> MSMEKQVLKENMKTTYHMDGSVDGHYFEIEGEGTGNPFKGEQELKLRVTKGGPLPFAFDILSPTFTYGNRVFTDYPEDMPDYFKQSLPEGYSWERTMMYEDGATATASARISLDKNGFVHKSTFHGENFPANGPVMKKKGVDWEPSSETITPEDGILKGDVEMFLVLEGGQRLKALFQTTYKANKVVKMPPR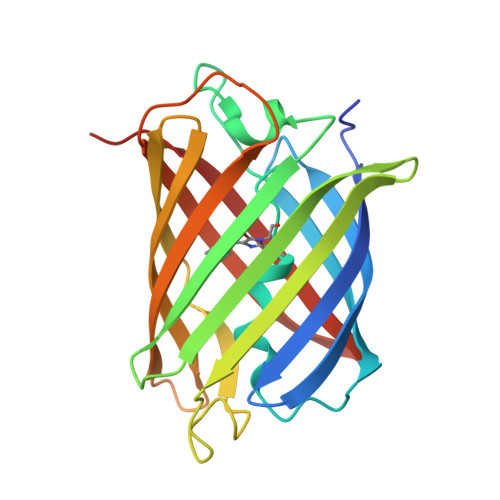HKIEHRLVRSEDGETIQLQEHAVAKYFTE Wzi, an integral outer-membrane protein from Escherichia coli, has been implicated in the formation of group 1 capsules. We conclude that Wzi is a novel outer-membrane lectin that assists in the formation of the bacterial capsule via direct interaction with capsular polysaccharides. Group 1 capsule-producing strains of E. coli secrete CPS into the extracellular environment when the wzi gene is knocked out, with the remaining cell-associated CPS unable to form a coherent capsule layer (Rahn et al., 2003). We propose that Wzi exposed on the surface of the cell acts as a lectin to bind to nascent EPS as it leaves the cell through the Wza translocase.

The 2.6 Å resolution structure of Wzi reveals an 18-stranded β-barrel fold with a novel arrangement of long extracellular loops that blocks the extracellular entrance and a helical bundle that plugs the periplasmic end. The X-ray structure reveals Wzi to be an 18-stranded antiparallel β-barrel, with the wall of the barrel describing a circle approximately 36 Å in diameter. Visual inspection and analysis with PISA indicates that Wzi is a monomer. The first-ordered residue is A24 (residues 1–23 are the cleaved signal peptide) and the last-ordered residue is L477 (C terminus of the mature protein). Not seen are residues 275–287, which form part of an extended loop between β9 and β10 (loop L5) and the C-terminal His tag. The barrel has a striking α-helical bundle (α1-3) that precedes the N-terminus of the first strand. The long extracellular loops—L3, L5, and L7—adopt distinct structures, parts of which fold into the barrel, whereas loops L5, L6, and L7 extend beyond the circumference of the barrel wall. The other loops are folded into the barrel and completely occlude the pore (PoreWalker [Pellegrini-Calace et al., 2009]). The lengths of the β strands are irregular; β4 is only six residues long and results in a triangular “notch” at the extracellular face of the barrel. Loops L3, L6, and L7 pack together to form a complex, positively charged electrostatic surface consistent with binding of the negatively charged sugar.

> AGLVVNDNDLRNDLAWLSDRGVIHLSLSTWPLSQEEIARALKKAKPSYSSEQVVLARINQRLSALKADFRVTGYTSTDQPGTPQGFGQTQPADNSLGLAFNNSGEWWDVHLQGNVEGGERISNGSRFNANGAYGAVKFWNQWLSFGQVPQWWGPGYEGSLIRGDAMRPMTGFLMQRAEQAAPETWWLRWVGPWQYQISASQMNQYNAVPHAKIIGGRFTFSPIQSLELGASRIMQWGGKGRPESLSNFWDGLTGKDNTAANDPNEPGNQLAGFDFKFKLEPTLGWPVSFYGQMIGEDESGFLPSANMFLGGIEGHHGWGKDAVNWYLEAHDTRTNMSRTNYSYTHHIYKDGYYQQGYPLGDAMGGDGQLVAGKVELITEDNQRWSTRLVYAKVNPENQSINKAFPHADTLKGIQLGWSGDVYQSVRLNTSLWYTNANNSDSDDVGASAGIEIPFSL>QRWVQFMKEAGQGSRDMWRAYSDMKKANWKNSDKYFHARGNYDAARRGPGGAWAAKVISDAREAVQKFTGHGAEDSRADQFANEWGRSGKDP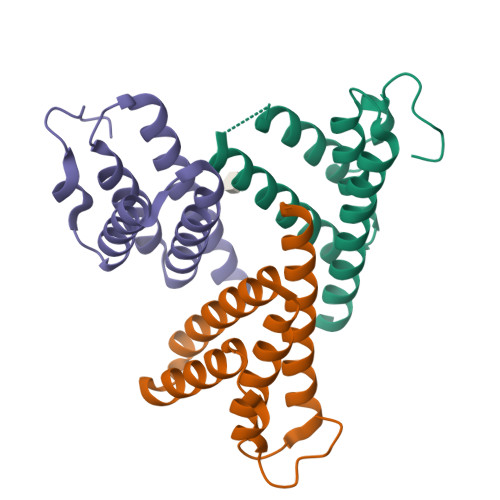NHFRPAGLPKRY[3x]The family of ρ-type GABAA receptors includes potential therapeutic targets in several neurological conditions, and features distinctive pharmacology compared to other subtypes. Channels in this family share a common architecture, with each of the five subunits contributing to an extracellular domain (ECD) with 10 strands (β1–β10) and a transmembrane domain (TMD) with 4 helices (M1–M4). The orthosteric ligand-binding site is located at the subunit interface in the ECD, composed of loops A, B and C from the principal subunit and D, E and F from the complementary subunit. We implemented a modified human ρ1 GABAA receptor construct (ρ1-EM) with truncated loops in the N-terminus and intracellular domain and an inserted fluorescent protein to facilitate expression while largely preserving wild-type function.

CGP36742 was the first GABAB receptor antagonist in clinical trials, but is also an orally active antagonist of ρ-type GABAA receptors, and has shown therapeutic potential for the treatment of cognitive deficits. In Xenopus laevis oocytes expressing ρ1-EM, THIP and CGP36742 antagonized GABA activation, consistent with previous studies of wild-type channels. In our cryo-EM structure, CGP36742 adopted an elongated pose, with its aminopropyl tail forming a salt bridge with E217 and cation-π interactions with the aromatic cage on the principal subunit face. The central phosphinic acid group was wedged between loop C on the principal subunit (making polar interactions with S264 and T265) and residue R125 on the complementary subunit, with the butyl tail extending toward the complementary β5 strand. The complex was comparable to the apo and THIP structures, and superimposable with our previous structure with TPMPA (Cα RMSD 0.035 Å), including analogous interactions of the amino and phosphinic acid groups; the additional butyl tail only required an alternative rotamer of M177 in the β5 strand. As in the case of TPMPA, the bulky, electronegative phosphinic acid group appeared to prevent lockdown of loop C over the antagonist, indicating a shared mechanism as well as binding pose among phosphinic acid inhibitors. The CGP36742 pose from our ρ1-EM structure could be placed in this pocket in the GABAB receptor complex by superposition on its equivalent aminopropyl and phosphinic acid moieties, or by computational docking, with similar poses showing no evident clashes and a favorable binding energy score. Interestingly, the amino group of CGP36742 was oriented roughly opposite to that of CGP35348 in its resolved site, indicating the rotational flexibility of these compounds could support their polymodal activities. Among phosphinic acid inhibitors, lockdown is obstructed by a consistent binding pose of CGP36742 and TPMPA, and likely of the subtype-specific agent (S)−4-ACPBPA.

>[5x]MLAVPNMRFGIFLLWWGWVLATESRMHWPGREVHEMSKKGRPQRQRREVHEDAHKQVSPILRRSPDITKSPLTKSEQLLRIDDHDFSMRPGFGGPAIPVGVDVQVESLDSISEVDMDFTMTLYLRHYWKDERLSFPSTNNLSMTFDGRLVKKIWVPDMFFVHSKRSFIHDTTTDNVMLRVQPDGKVLYSLRVTVTAMCNMDFSRFPLDTQTCSLEIESYAYTEDDLMLYWKKGNDSLKTDERISLSQFLIQEFHTTTKLAFYSSTGWYNRLYINFTLRRHIFFFLLQTYFPATLMVMLSWVSFWIDRRAVPARVPLGITTVLTMSTIITGVNASMPRVSYIKAVDIYLWVSFVFVFLSVLEYAAVNYLTTVQERKEQKLREKLPCTSGLPPPRTAMLDGNYSDGEVNDLDNYMPENGEKPDRMMVQLTLASERSSPQRKSQRSSYVSMRIDTHAIDKYSRIIFPAAYILFNLIYWSIFS[1-(3,4-dichlorophenyl)-1,2,3-triazol-4-yl]methanol | C9 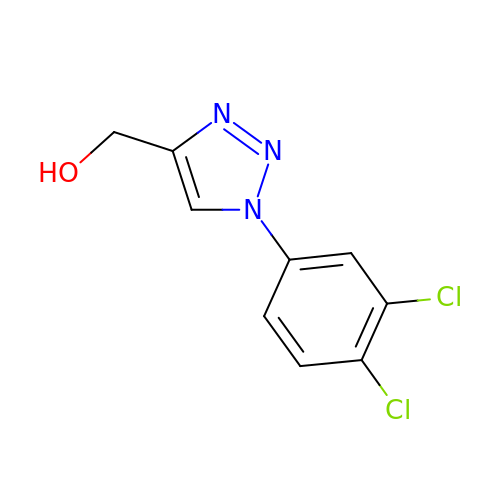H7 Cl2 N3 O | DMIRTDWEKUNBDX-UHFFFAOYSA-N>[2x]MAPTQLDIKV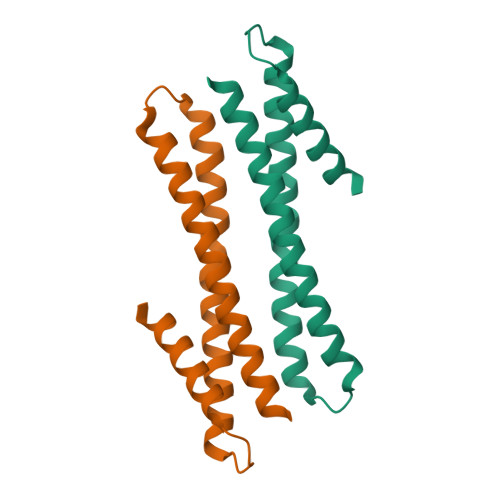KALKRLTKEEGYYQQELKDQEAHVAKLKEDKSVDPYDLKKQEEVLDDTKRLLPTLYEKIREFKEDLEQFLKTYQGTEDVSDARSAITSAQELLDSK> AFEDRDPTQFEERHLKFLQQLGKGNFGSVEMCRYDPLQDNTGEVVAVKKLQHSTEEHLRDFEREIEILKSLQHDNIVKYKGVCYSAGRRNLKLIMEYLPYGSLRDYLQKHKERIDHIKLLQYTSQICKGMEYLGTKRYIHRDLATRNILVENENRVKIGDFGLTKVLPQDKEYYKVKEPGESPIFWYAPESLTESKFSVASDVWSFGVVLYELFTYIEKSKSPPAEFMRMIGNDKQGQMIVFH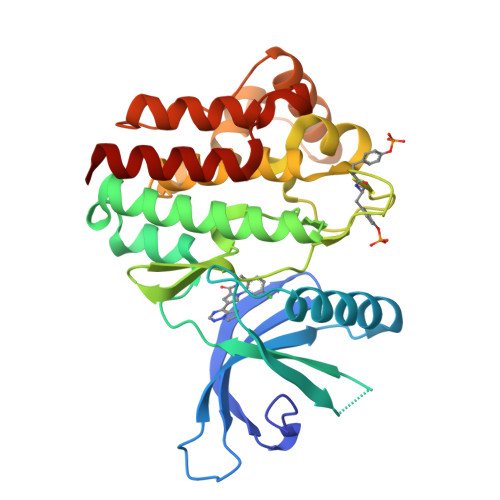LIELLKNNGRLPRPDGCPDEIYMIMTECWNNNVNQRPSFRDLALRVDQIRDNMAG StnA is an essential enzyme in the Streptonigrin biosynthesis pathway. The crystal structure shows that StnA has an α-helical cap domain positioned atop a common α/β hydrolase domain. The data clearly shows that Ser185-Asp308-His349 constitutes the catalytic triad of StnA.

The selenomethionine substituted StnA (SeMet-StnA) was crystallized in the space group C2 with four molecules per asymmetric unit. The structure of the enzyme was determined by single-wavelength anomalous dispersion (SAD) phasing method and refined to 2.71 Å with an Rfactor of 0.1923 and Rfree of 0.2196. The final model of StnA consists of residues 61–375 because of the poor electron density for the 60 residues at the N-terminal region. Residue Thr77 in each monomer is in the cis conformation. StnA is stabilized by two additional disulfide bonds of Cys61/Cys64 and Cys312/Cys319, which are located between β1 and β2 and between β7 and αD, respectively. The catalytic His349, located in the loop between β8 and helix αF, points towards the nucleophile, with its Nε2 atom at a distance of 3.2 Å from the Oγ atom of Ser185. The His349 Nδ1 atom forms a hydrogen bond/salt bridge with Oδ1 (3.2 Å) and Oδ2 (2.7 Å) of Asp308, located between strand β7 and helix αE. The overall structures of the free and complex are very similar with a RMSD of 0.232 Å over 316 Cα atoms.

>VTALSRLGEPPSGHDGNSEVRRIAMKRATVPVLRRVAAVCAAALLVTVGTGGPASATGTRSAICRATTVEVTLGKGTGKMWGELCRPAGSSPDTVVTMVHGATYNHNYWDFPYQPDKYSFRKMLNGAGYATFVVDRLGTGNSTVPPSSELNLTVEARQMHEVVQGLRTGRIGGTGFGKVVLAGYSLGSAVTSIEASTFHDVDAVLITALGHYNNPAGTQAIIDNGLSPNDDPVLKDRHHYDDGYATTKPGSRKHVFYADRPMDPGVLATDELTKDANVFTEAADPLVIDPAVSRAIDVPVMFALGDRDPLMCGDGYEDCSSQAALRAQEAPFWTSAPSFDVILVEDAGHGLNLVPNTRVYQDASRDWLDRVVGHGLEHHHHHH[4x]> MEKLFTGDIMEIQNTKVDSAFMKNKIVPYKGTTTLAFIFQGGMVIAVDSRASAGSYIASQNVHKVIRVNKHLIGTMAGGASDCYFWEKKMGLYAKLYELKNNKRISVSAASMYLSNCVYSYKGQGLSLGSMVCGYDGDKPVIYYVDDAGQRLSGDLF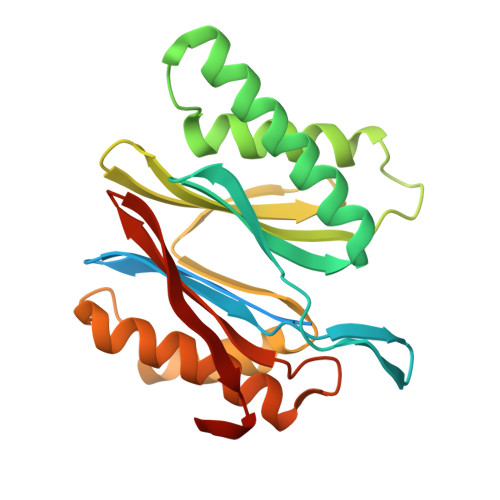SVGSGSTIAYGVLNESYRFDLTKEEALNLGKKAIWHATHRDAYSGGNVNLYFMDKNGWEHLGTFDVDKFEQ N~2~-({(1R,2R,3S)-2-(methylcarbamoyl)-3-[4-(phosphonooxy)phenyl]cyclopropyl}carbonyl)-D-glutaminyl-D-aspartamide 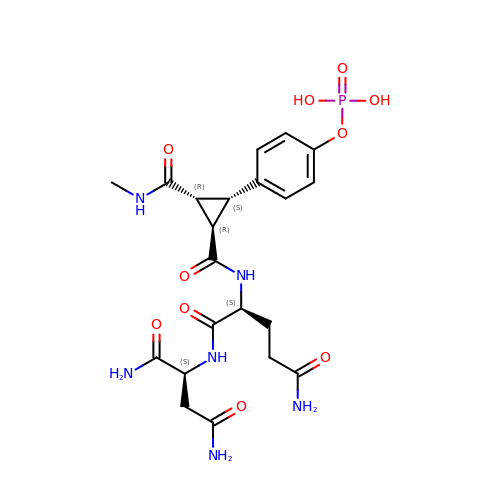| C21 H29 N6 O10 P | RYXSIJXAOLAGQV-PASATYPHSA-N> ASMGKSAVIFVERATPATLTELKDALSNSILSVRDPWSIDFRTYRCSIKNLPADVSKLMYSITFHHHGRQTVLIKDNSAMVTTAAAADIPPALVFNGSSTGVPESIDTILSSKLSNIWMQRQLIKGDAGETLILDGLTVRLVNLFSS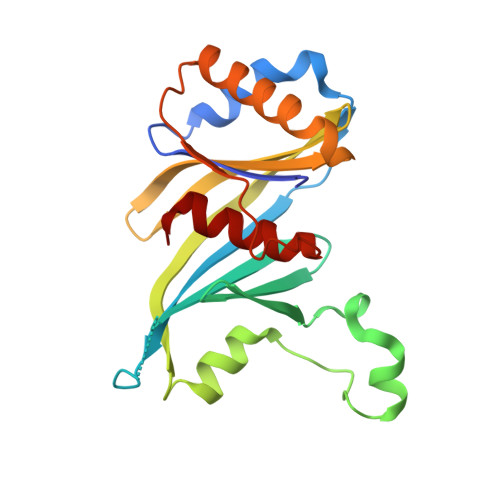TGFKGLLIELQADEAGEFETKIAGIEGHLAEIRAKEYKTSSDSLGPDTSNEICDLAYQYVRALEL>[2x]MEF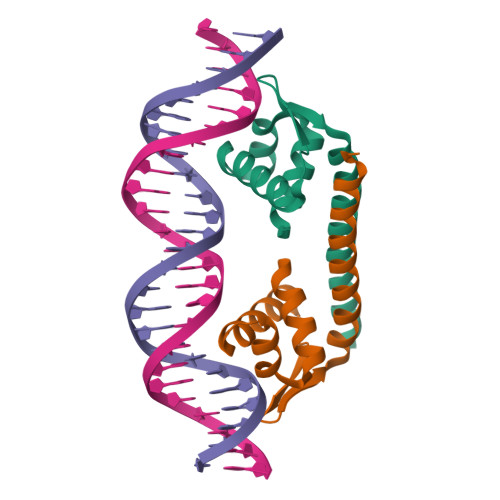RQLKYFIAVAEAGNMAAAAKRLHVSQPPITRQMQALEADLGVVLLERSHRGIELTAAGHAFLEDARRILELAGRSGDRSRAAARENLYFQGAHHHHHH>GAMDPGNSAEAWKNLGNAYYKQGDYQKAIEYYQKALELDPNNASAWYNLGNAYYKQGDYQKAIEYYQKALELDPNNAKAWYRRGNAYYKQGDYQKAIEDYQKALELDPNNAKAKQNLGNAKQKQG[5x];>[5x]XME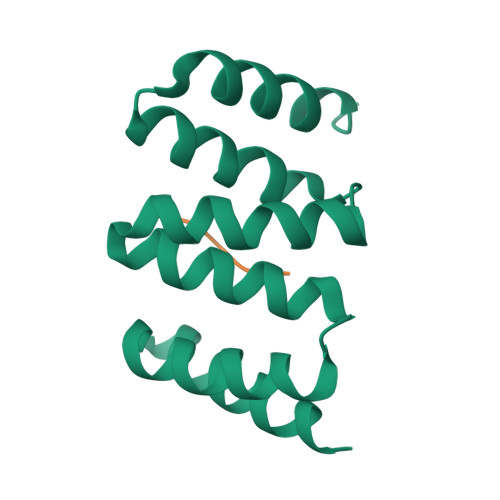EVD> GSAKDPMRVLKYAILGLLRKGELSGYDITSYFKEELGQFWSAKHSQIYPELKKLTDEGFITFRTTIQGTKLEKKMYTLTDSGKQELHDWLIRHQPIPETVKDEFMLKAYFISSLSRQEASDLFTDQLLKRKAKLSDLQGSYEKLMASAEPMS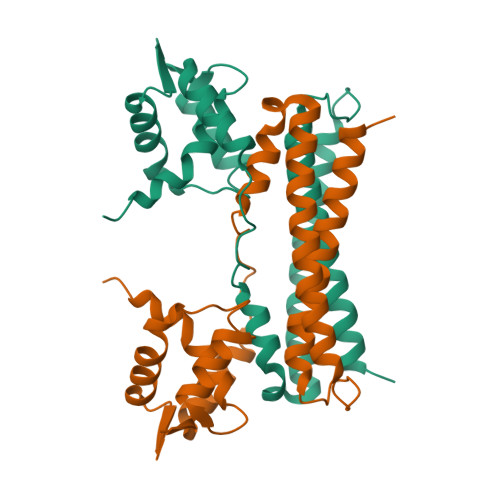FSSPDFGHYLVLTKALEREKNYVSWLESILAMIDED>[2x]SVRIQVINPNTSLAMTETIGAAARAVAAPGTEILAVCPRAGVPSIEGHFDEAIAA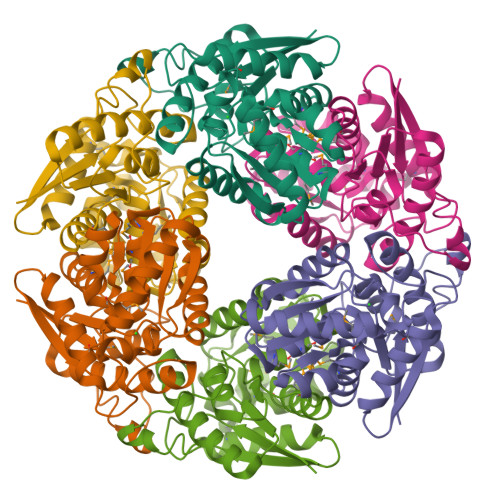VGVLEQIRAGREQGVDGHVIACFGDPGLLAARELAQGPVIGIAEAAMHMATMVATRFSIVTTLPRTLIIARHLLHQYGFHQHCAALHAIDLPVLALEDGSGLAQEKVRERCIRALKEDGSGAIVLGCGGMATLAQQLTRELRVPVIDGVSAAVKMVESLVALGLATSKHGDLAFPEKKALSGQFQSLNPF AGT is a hepatocyte-specific PLP dependent enzyme, belonging to the Fold Type I family, catalysing the transamination reaction between L-alanine and glyoxylate to produce glycine and pyruvate, thus leading to the removal of glyoxylate. AGT normally localises in the peroxisomes and failure of its detoxification role leads to increased levels of oxalate, coming from oxidation of glyoxylate, causing calcium oxalate precipitation in the kidney and urinary tract. Many pathogenic variants of AGT cause PH1 (primary hyperoxaluria type I), a rare autosomal recessive disorder. Our results shows that two forces generated by the salt bridge between the conserved aspartate residue and the pyridine N1 atom, and by the Schiff base linkage act as opposite springs and are responsible for the fine tilting adjustments of the pyridine plane of PLP.

D183N is a pathogenic variant of AGT that causes Primary Hyperoxaluria Type I (PH1), a severe disorder of glyoxylate metabolism. Although the mutation is conservative, the variant shows a 2.3 × 104 fold reduction of the catalytic efficiency, whereas the affinity for PLP is almost unchanged. By coupling this result with the crystal structure at different pH of the AGT pathogenic variant D183N, bearing the mutation of the conserved aspartate, and with a molecular dynamic simulation of the transaldimination step, we propose a novel interpretation of the conserved aspartate role. While the wild type enzyme at pH > 7.5 shows spectral changes, which can be interpreted as deprotonation of the internal aldimine, in the mutant the internal aldimine is protonated over a wide range of pH values (5.0–9.2). This effect is also a consequence of the strain relaxation, which increases the stability of the protonated species. The strain release of the D183N mutant is also likely responsible for the slight increase in thermal stability observed for this variant, and for its apparent resistance towards radiation damage, given that the internal aldimine of the mutant seems not to undergo x-ray induced-reduction both at acidic and alkaline pH.

> MASHKLLVTPPKALLKPLSIPNQLLLGPGPSNLPPRIMAAGGLQMIGSMSKDMYQIMDEIKEGIQYVFQTRNPLTLVISGSGHCALEAALVNVLEPGDSFLVGANGIWGQRAVDIGERIGARVHPMTKDPGGHYTLQEVEEGLAQHKPVLLFLTHGESSTGVLQPLDGFGELCHRYKCLLLVNSVASLGGTPLYMDRQGIDILYSGSQKALNAPPGTSLISFSDKAKKKMYSRKTKPFSFYLDIKWLANFWGCDDQPRMYHHTIPVISLYSLRESLALIAEQGLENSWRQHREAAAYLHGRLQALGLQLFVKDPALRLPTVTTVAVPAGYDWRDIVSYVIDHFDIEIMGGLGPSTGKVLRIGLLGCNATRENVDRVTEALRAALQHCPKKKL>[4x]MDHHHHHHLPNITILATGGTIAGGGDSATKSNYTVGKVGVENLVNAVPQLKDIANVKGEQVVNIGSQDMNDNVWLTLAKKINTDCDKTDGFVITHGTDTMEETAYFLDLTVKC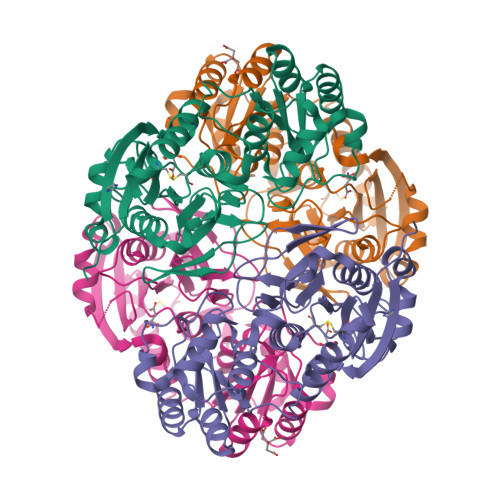DKPVVMVGAMRPSTSMSADGPFNLYNAVVTAADKASANRGVLVVMNDTVLDGRDVTKTNTTDVATFKSVNYGPLGYIHNGKIDYQRTPARKHTSDTPFDVSKLNELPKVGIVYNYANASDLPAKALVDAGYDGIVSAGVGNGNLYKSVFDTLATAAKTGTAVVRSSRVPTGATTQDAEVDDAKYGFVASGTLNPQKARVLLQLALTQTKDPQQIQQIFNQY> GPGS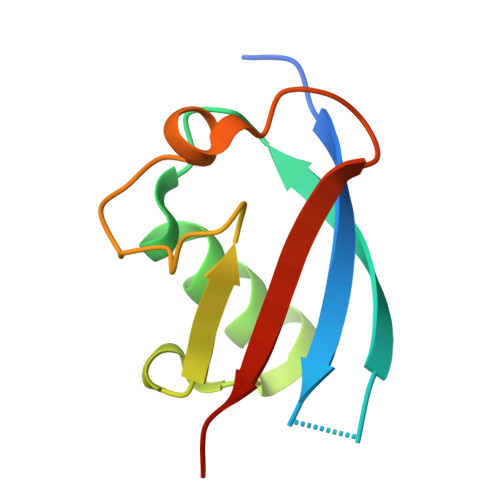EFQDIRLWVSVEDAQMHTVTIWLTVRPDMTVASLKDMVFLDYGFPPVLQQWVIGQRLARDQETLHSHGVRQNGDSAYLYLLSARN>MIDFGNFYSLIAKNHLSHWLETLPAQIANWQREQQHGLFKQWSNAVEFLPEIKPYRLDLLHSVTAESEEPLSAGQIKRIETLMRNLMPWRKGPFSLYGVNIDTEWRSDWKWDRVLPHLSDLTGRTILDVGCGSGYHMWRMIGAGAHLAVGIDPTQLFLCQFEAVRKLLGNDQRAHLLPLGIEQLPALKAFDTVFSMGVLYHRRSPLEHLWQLKDQLVNEGELVLETLVIDGDENTVLVPGDRYAQMRNVYFIPSALALKNWLKKCGFVDIRIADVSVTTTEEQRRTEWMVTESLADFLDPHDPGK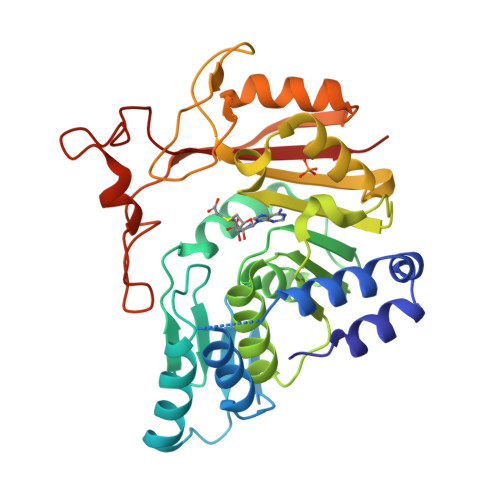TVEGYPAPKRAVLIARKP[2x]> G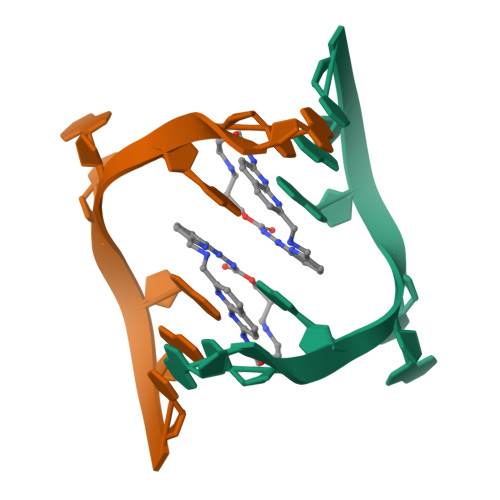CAGCAGC>MTGGMKPPARKPRILNSDGSSNITRLGLEKRGWLDDHYHDLLTVSWPVFITLITGLYLVTNALFALAYLACGDVIENARPGSFTDAFFFSVQTMATIGYGKLIPIGPLANTLVTLEALCGMLGLAVAASLIYARFTRPTAGVLFSSRMVISDFEGKPTLMMRLANLRIEQIIEADVHLVLVRSEISQEGMVFRRFHDLTLTRSRSPIFSLSWTVMHPIDHHSPIYG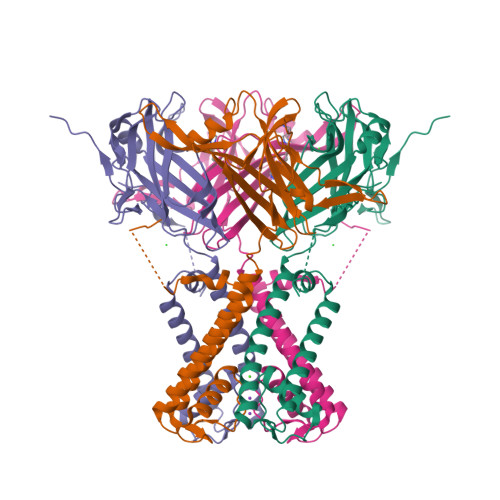ETDETLRNSHSEFLVLFTGHHEAFAQNVHARHAYSCDEIIWGGHFVDVFTTLPDGRRALDLGKFHEIAQHHHHHH[2x]> FQGAMSSSIDISKINSWNKE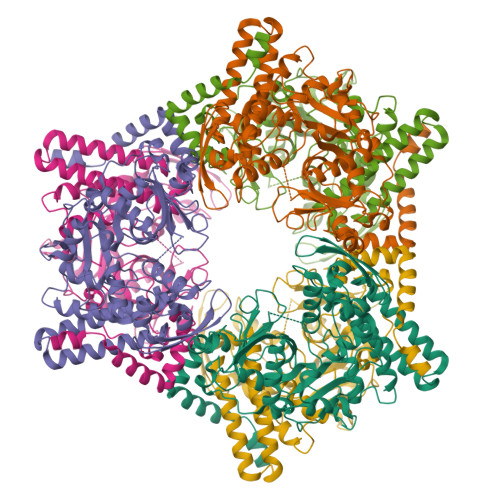FQSDLTHQLATTVLKNYNADDALLNKTRLQKQDNRVFNTVVSTDSTPVTNQKSSGRCWLFAATNQLRLNVLSELNLKEFELSQAYLFFYDKLEKANYFLDQIVSSADQDIDSRLVQYLLAAPTEDGGQYSMFLNLVKKYGLIPKDLYGDLPYSTTASRKWNSLLTTKLREFAETLRTALKERSADDSIIVTLREQMQREIFRLMSLFMDIPPVQPNEQFTWEYVDKDKKIHTIKSTPLEFASKYAKLDPSTPVSLINDPRHPYGKLIKIDRLGNVLGGDAVIYLNVDNETLSKLVVKRLQNNKAVFFGSHTPKFMDKKTGVMDIELWNYPAIGYNLPQQKASRIRYHESLMTLAMLITGCHVDETSKLPLRYRVENSWGKDSGKDGLYVMTQKYFEEYCFQIVVDINELPKELASKFTSGKEEPIVLPIWDPMGALA> SLHMIDYK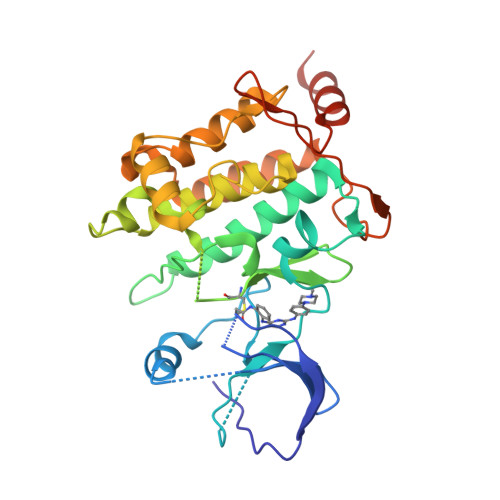EIEVEEVVGRGAFGVVCKAKWRAKDVAIKQIESESERKAFIVELRQLSRVNHPNIVKLYGACLNPVCLVMEYAEGGSLYNVLHGAEPLPYYTAAHAMSWCLQCSQGVAYLHSMQPKALIHRDLKPPNLLLVAGGTVLKICDFGTACDIQTHMTNNKGSAAWMAPEVFEGSNYSEKCDVFSWGIILWEVITRRKPFDEIGGPAFRIMWAVHNGTRPPLIKNLPKPIESLMTRCWSKDPSQRPSMEEIVKIMTHLMRYFPGADEPLQYPCQHSLPPGEDGRVEPYVDFAEFYRLWSVDHGEQSVVTAP>[2x]GHMKELWRQCTHWLIQCRVLPPSHRVTWEGAQVCELAQALRDGVLLCQLLNNLLPHAINLREVNLRPQMSQFLCLKNIRTFLSTCCEKFGLKRSELFEAFDLFDVQDFGKVIYTLSALSWTPIAQNRGIMPFPTEEESVGDEDIYSGLSDQIDDTVEEDEDLYDCVENEEAEGDEIYEDLMRSEPVSMPPKMTEYDKRCCCLREIQQTEEKYTDTLGSIQQHFLKPLQRFLKPQDIEIIFINIEDLLRVHTHFLKEMKEALGTPGAANLYQVFIKYKERFLVYGRYCS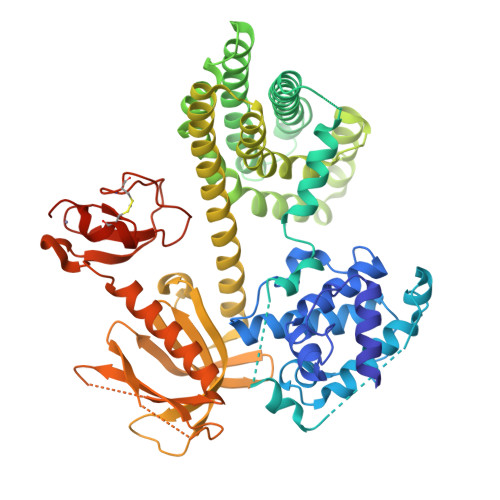QVESASKHLDRVAAAREDVQMKLEECSQRANNGRFTLRDLLMVPMQRVLKYHLLLQELVKHTQEAMEKENLRLALDAMRDLAQCVNEVKRDNETLRQITNFQLSIENLDQSLAHYGRPKIDGELKITSVERRSKMDRYAFLLDKALLICKRRGDSYDLKDFVNLHSFQVRDDSSGDRDNKKWSHMFLLIEDQGAQGYELFFKTRELKKKWMEQFEMAISNIYPENATANGHDFQMFSFEETTSCKACQMLLRGTFYQGYRCHRCRASAHKECLGRVPPCGRHGQDFPGTMKKDKLHRRA> LLGDFFRKSKEKIGKEFKRIVQRIKDFLRNLVPRTES

LL-37 is an extensively studied peptide with particular relevance in human innate immunity. LL-37 is produced as a precursor protein in human cells (e.g. leukocytes or neutrophils) and processed during its secretion to the skin, lungs, or reproductive tract. The active peptide carries a surplus of positive charge, which is attributed to interactions with the LPS or LTA of the bacterial cell wall, and negatively charged lipids of in vivo cytoplasmic membranes. We determined its atomic structure in solution and the putative membrane interaction states. Together the structures in the absence and presence of detergents revealed discrete detergent binding sites at the dimer interface indicating the presence of in vivo lipid binding sites.

Our first crystals yielded a monomeric structure at atomic resolution (termed LL-37DPC-1) obtained under conditions comprising artificially high MPD concentrations (70% MPD). The second structure (termed LL-372) obtained in the absence of detergents displays an anti-parallel dimer formed by two α-helices without supercoiling. The monomers are identical to LL-37DPC-1 with each amphipathic helix extending to ~5 nm. Intramolecular stabilization of the monomer is provided by backbone H-bonds and salt bridges (formed between Asp4 and Arg7, Glu16 and Arg19 and Asp26 and Arg29, Gln22 and Asp26).> MPDTSFSNPGLFTPLQLGSLSLPNRVIMAPLTRSRTPDSVPGRLQQIYYGQRASAGLIISEATNISPTARGYVYTPGIWTDAQEAGWKGVVEAVHAKGGRIALQLWHVGRVSH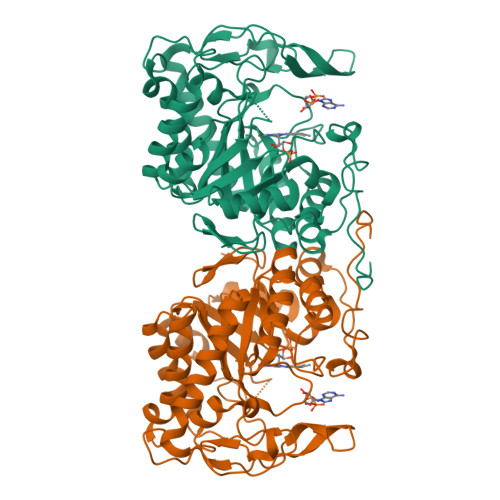ELVQPDGQQPVAPSALKAEGAECFVEFEDGTAGLHPTSTPRALETDEIPGIVEDYRQAAQRAKRAGFDMVEVHAAAACLPNQFLATGTNRRTDQYGGSIENRARFPLEVVDAVAEVFGPERVGIRLTPFLELFGLTDDEPEAMAFYLAGELDRRGLAYLHFNEPDWIGGDITYPEGFREQMRQRFKGGLIYCGNYDAGRAQARLDDNTADAVAFGRPFIANPDLPERFRLGAALNEPDPSTFYGGAEVGYTDYPFLDNGHDRLG> GAMGYKDNIRHGVCWIYYPDGGSLVGEVNEDGEMTGEKIAYVYPDERTALYGKFIDGEMIEGKLATLMSTEEGRPHFELMPGNSVYHFDKSTSSCISTNALLPDPYESERVYVAESLISSAGEGLFSKVAVGPNTVMSFYNGVRITH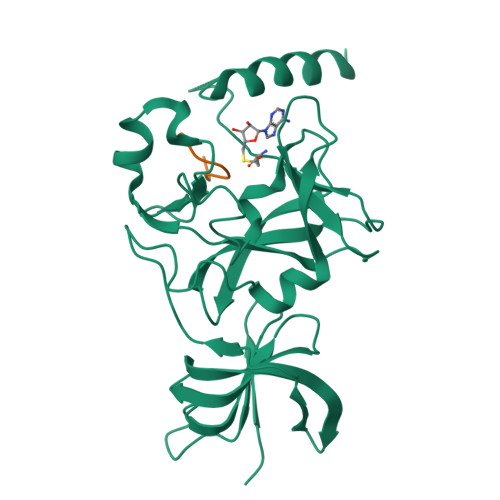QEVDSRDWALNGNTLSLDEETVIDVPEPYNHVSKYCASLGHKANHSFTPNCIFDMFVHPRFGPIKCIRTLRAVEADEELTVAYGYDHSPPGKSGPEAPEWYQVELKAFQATQQK;> XSKSKDRKYTL> MGIDINTKIFNSVAEVFQKAQGSYAGHRKHIAVLKKIQSKAVEQGYEDAFNFWFDKLVTKILPLKKNEIIGDRIVKLVAAFIASLERELILAKKQNYKLTNDEEGIFSRFVDQFIRHVLRGVESPDKNVRFRVLQLLAVIMDNIGEIDESLFNLLILSLNKRIYDREPTVRIQAVFCLTKFQDEEQTEHLTELSDNEENFEATRTLVASIQNDPSAEVRRAAMLNLINDNNTRPYILERARDVNIVNRRLVYSRILKSMGRKCFDDIEPHIFDQLIEWGLEDRELSVRNACKRLIAHDWLNALDGDLIELLEKLDVSRSSVCVKAIEALFQSRPDILSKIKFPESIWKDFTVEIAFLFRAIYLYCLDNNITEMLEENFPEASKLSEHLNHYILLRYHHNDISNDSQSHFDYNTLEFIIEQLSIAAERYDYSDEVGRRSMLTVVRNMLALTTLSEPLIKIGIRVMKSLSI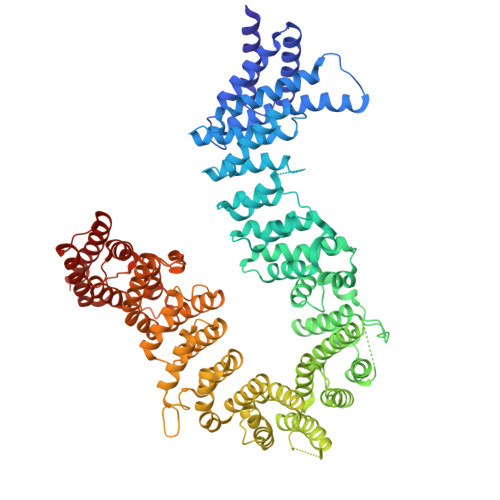NEKDFVTMAIEIINDIRDDDIEKQESESDIINNLPPEKEASSATIVLCLTRSSYMLELVNTPLTENILIASLMDTLITPAVRNTAPNIRELGVKNLGLCCLLDVKLAIDNMYILGMCVSKGNASLKYIALQVIVDIFSVHGNTVVDGEGKVDSISLHKIFYKVLKNNGLPECQVIAAEGLCKLFLADVFTDDDLFETLVLSYFSPINSSNEALVQAFAFCIPVYCFSHPAHQQRMSRTAADILLRLCVLWDDLQSSVIPEVDREAMLKPNIIFQQLLFWTDPRNLVNQTGSTKKDTVQLTFLIDVLKIYAQIEKKEIKKMIITNINAIFLSSEQDYSTLKELLEYSDDIAENDNLDNVSKNALDKLRNNLNSLIEEINERSETQTKDENNTANDQYSSILGN> MTLNRKCVVIHNGSHRTVAGFSNVELPQCIIPSSYIKRTDEGGEAEFIFGTYNMIDAAAEKRNGDEVYTLVDSQGLPYNWDALEMQWRYLYDTQLKVSPEELPLVITMPATNGKPDMAILERYYELAFDKLNVPVFQIVIEPLAIALSMGKSSAFVIDIGASGCNVTPIIDGIVVKNAVVRSKFGGDFLDFQVHERLAPLIKEENDMENMADEQKRSTDVWYEASTWIQQFKSTMLQVSEKDLFELERYYKEQADIYAKQQEQLKQMDQQLQYTALTGSPNNPLVQKKNFLFKPLNKTLTLDL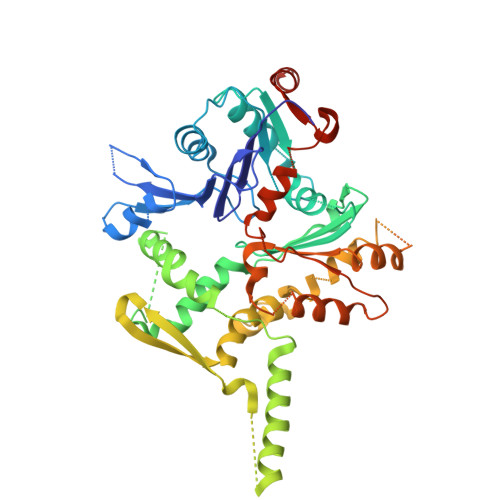KECYQFAEYLFKPQLISDKFSPEDGLGPLMAKSVKKAGASINSMKANTSTNPNGLGTSHINTNVGDNNSTASSSNISPEQVYSLLLTNVIITGSTSLIEGMEQRIIKELSIRFPQYKLTTFANQVMMDRKIQGWLGALTMANLPSWSLGKWYSKEDYETLKRDRKQSQATNATN Here, we demonstrate that reduced form of damavaricin C as a vital precursor is finally transformed into MDB-contained mature streptovaricins (streptovaricin C and streptovaricin B or J) by cytochrome P450 enzyme StvP2 after sequential methylation and acetylation. As a result, a component whose retention time, UV/Vis (ultraviolet–visible) spectrum and m/z value are well consistent with 1 was produced (yield > 98%) giving a direct evidence for the function of StvP2 to catalyze MDB formation in mature streptovaricins. To enhance our understanding of MDB formation by StvP2, we solved the X-ray crystal structure of StvP2 at 1.35 Å resolution and the StvP2 in complex with substrate 2 at 2.3 Å resolution, respectively. The overall crystal structures of substrate-free and substrate-bound StvP2 adopts a typical P450 fold, consisted of twelve α-helices (A–L) and two β-sheets (1–2), with a heme as the core cofactor.

The I helix, BC loop, the loop following the K helix, the second β strand of β 1 sheet and C-terminal residues together constructs a large substrate binding cavity by comparison of substrate-free and substrate-bound structures. The conformation of substrate-bound StvP2 structure showed no significant changes relative to the substrate-free StvP2 structure.

> MTETPATPTGLPTARAAGCPFDPPPGLAALRDRAPLTRMEFPNGHVGWLATGHAVVRAVLADPRFSHRNDRRHWPLADIGRGFPPLPGDMLHIDPPDHTRYRKLLAGKFTMRRMRRLTGSAQEIVAGKLDAMERHGGPLDLLEFFARPVPTLMVCALLGVPLQDRATFHPPVRGTDDAAAVEADVAAYVEMTYADMQEYFRKLVAAKRAAPADDLLSDLTTSDLTEDELVGLCAVMMHAGVDSTSNMLALGTWALLERPDQLAALRERPDLADRAVEELMRYMSVVHTGSRAALEDVELAGEVVRAGESVAFSVQAANRDPARFADPDTLDIRRGAVGHLGFGYGVHQCLGMQLARVEMRVAFPALFARFPALRLAVPAGDVPMRDDLVIPYGVHRLPVTW> GSHMVLTK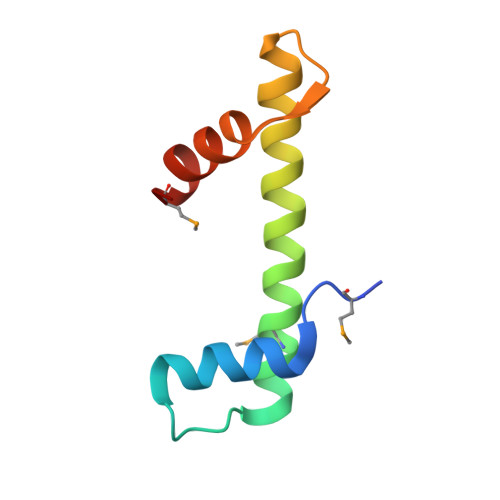KKLQDLVREVDPNEQLDEDVEEMLLQIADDFIESVVTAACQLARHRKSSTLEVKDVQLHLERQWNMWI> SRLIFEHQRRLTPPTTRKGTITIEPPPQLPRVVPPSLLRRVLPFLIVILIVGMIVALFATGMRL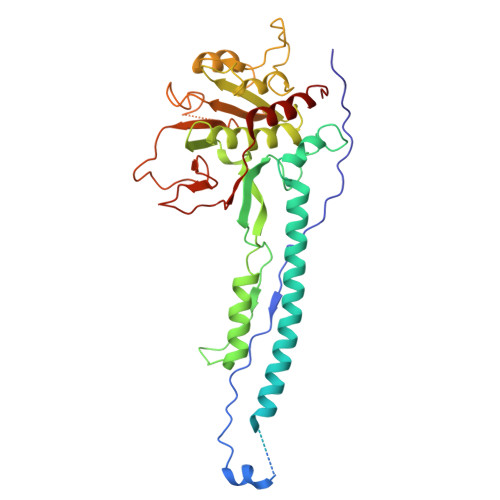ISPTMLFFPFVLLLAATALYRGGDNKMRTEEVDAERADYLRYLSVVRDNVRAHAAEQRAALEWSHPEPEVLATIPGTRRQWERDPRDRDFLVLRAGRHDVPLDAALKVKDTADEIDLEPVAHSALRGLLDVQRTVRDAPTGLDVAKLARITVIGEADEARAAIRAWIAQAVTWHDPTMLGVALAAPDLESGDWSWLKWLPHVDVPNEADGVGPARYLTTSTAELRERLAPALADRPLFPAESGAALKHLLVVLDDPDADPDDIARKPGLTGVTVIHRTTELPNREQYPDPERPILRVADGRIERWQVGGWQPCVDVADAMSAAEAAHIARRLSRWDS>ILGGTEAEEGSWPWQVSLRLNNAHHCGGSLINNMWILTAAHCFRSNSNPRDWIATSGISTTFPKLRMRVRNILIHNNYKSATHENDIALVRLENSVTFTKDIHSVCLPAATQNIPPGSTAYVTGWGAQEYAGHTVPELRQGQVRIISNDVCNAPHSYNGAILSGMLCAGVPQGGVDACQGDAGGPLVQEDSRRLWFIVGIVSWGDQCGLPDKPGVYTRVTAYLDWIRQQTGI[2x];>[2x]LINECGAGPDL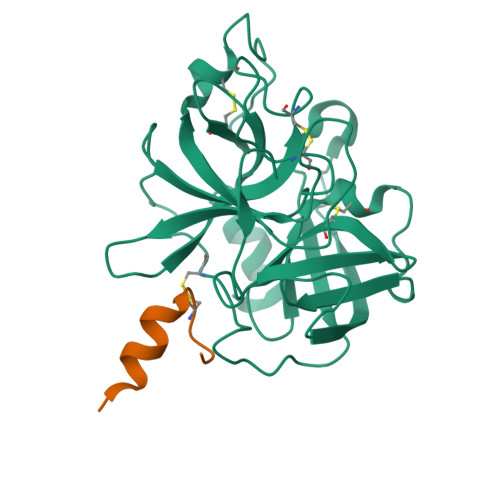ITLSEQR> QYVRIKNWGSGEI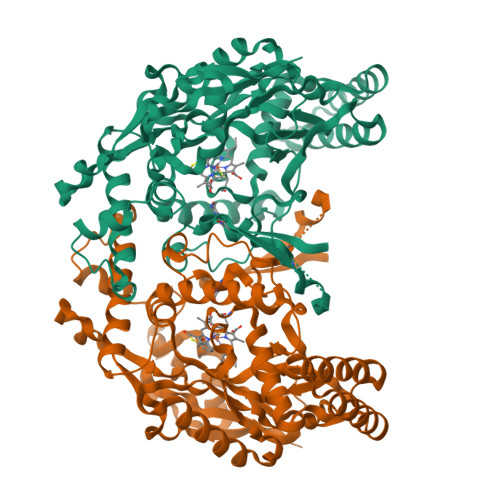LHDTLHHKATSDFTCKSKSCLGSIMNPKSLTRGPRDKPTPLEELLPHAIEFINQYYGSFKEAKIEEHLARLEAVTKEIETTGTYQLTLDELIFATKMAWRNAPRCIGRIQWSNLQVFDARNCSTAQEMFQHICRHILYATNNGNIRSAITVFPQRSDGKHDFRLWNSQLIRYAGYQMPDGTIRGDAATLEFTQLCIDLGWKPRYGRFDVLPLVLQADGQDPEVFEIPPDLVLEVTMEHPKYEWFQELGLKWYALPAVANMLLEVGGLEFPACPFNGWYMGTEIGVRDFCDTQRYNILEEVGRRMGLETHTLASLWKDRAVTEINVAVLHSFQKQNVTIMDHHTASESFMKHMQNEYRARGGCPADWIWLVPPVSGSITPVFHQEMLNYVLSPFYYYQIEPWKTHIWQNE>[2x]GSHMGRRKRTAVTGSQTALLLRAFEKDRFPGIAAREELARETGLPESRIQIWFQNRR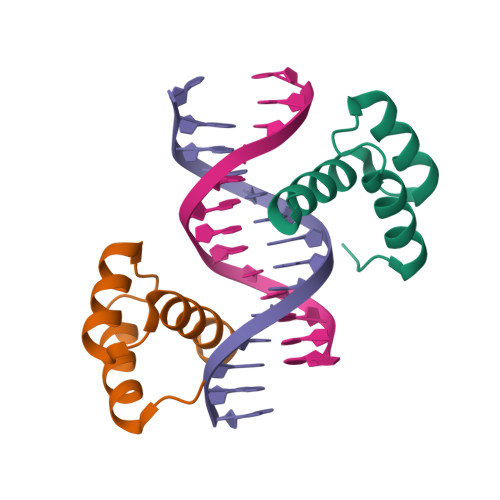ARHPGQG> ETGQPAQCRIQKCTTDFVSLTSHLNSAVDGFDSEFCKALRAYAGCTQRTSKACRGNL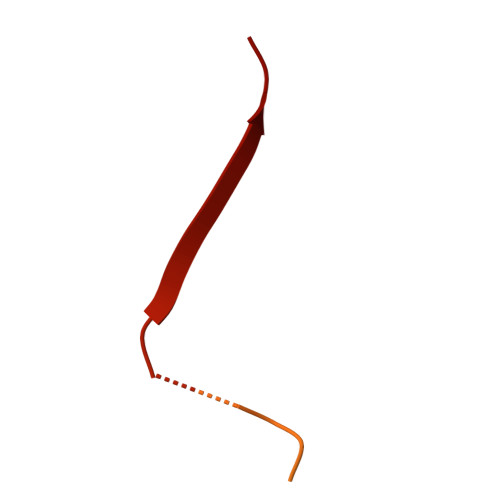VYHSAVLGISDLMSQRNCSKDGPTSSTNPEVTHDPCNYHSHAGAREHRRGDQNPPSYLFCGLFGD> GPLGSMASPEERLLDELNNVIVSFLCDSGSLEVERCSGAHVFSRGSSQPLCTVKLRHGQIYHLEFVYKFLAFKLKNCNYPSSPVFVISNNGLATTLR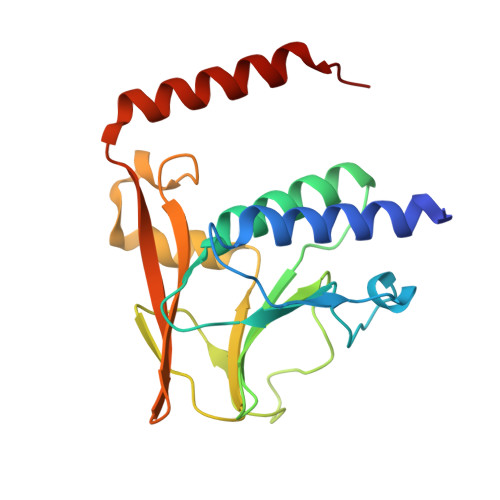CFLHEPSGLRSGQSGPCLGLSTDVDLPKNSIIMLGQDDFIKFKSPLVFPAELDLLKSMVVCRAYITEHRTTMQFLVFQAANAQKASRVMDMISDMSQQLSRSG>[3x]MKKILDSAKNYLNTHDKLKTACLIALELPSSSGSAATYIYLTDYFRDVTYNGILYRSGKVKSISSHKQNRQLSIGSLSFT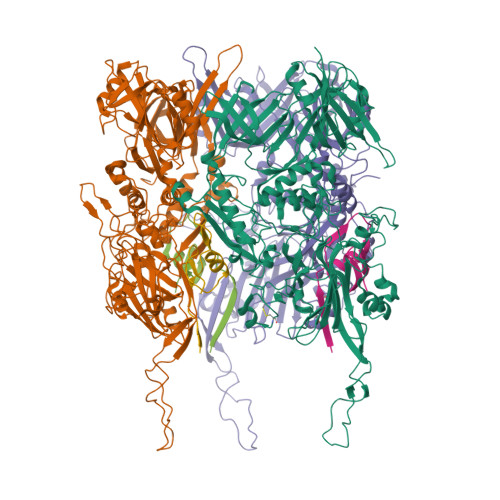ITGTAEDEVLKLVQNGVSFLDRGITIHQAIINEEGNILPVDPDTDGPLLFFRGRITGGGIKDNVNTSGIGTSVITWNCSNQFYDFDRVNGRYTDDASHRGLEVVNGTLQPSNGAKRPEYQEDYGFFHSNKSTTILAKYQVKEERYKLQSKKKLFGLSRSYSLKKYYETVTKEVDLDFNLAAKFIPVVYGVQKIPGIPIFADTELNNPNIVYVVYAFAEGEIDGFLDFYIGDSPMICFDETDSDTRTCFGRKKIVGDTMHRLAAGTSTSQPSVHGQEYKYNDGNGDIRIWTFHGKPDQTAAQVLVDIAKKKGFYLQNQNGNGPEYWDSRYKLLDTAYAIVRFTINENRTEIPEISAEVQGKKVKVYNSDGTIKADKTSLNGIWQLMDYLTSDRYGADITLDQFPLQKVISEAKILDIIDESYQTSWQPYWRYVGWNDPLSENRQIVQLNTILDTSESVFKNVQGILESFGGAINNLSGEYRITVEKYSTNPLRINFLDTYGDLDLSDTTGRNKFNSVQASLVDPALSWKTNSITFYNSKFKEQDKGLDKKLQLSFANITNYYTARSYADRELKKSRYSRTLSFSVPYKFIGIEPNDPIAFTYERYGWKDKFFLVDEVENTRDGKINLVLQEYGEDVFINSEQVDNSGNDIPDISNNVLPPRDFKYTPTPGGVVGAIGKNGELSWLPSLTNNVVYYSIAHSGHVNPYIVQQLENNPNERMIQEIIGEPAGLAIFELRAVDINGRRSSPVTLSVDLNSAKNLSVVSNFRVVNTASGDVTEFVGPDVKLAWDKIPEEEIIPEIYYTLEIYDSQDRMLRSVRIEDVYTYDYLLTYNKADFALLNSGALGINRKLRFRIRAEGENGEQSVGWATI;>MTDKLIRELLIDVKQKGATRTAKSIENVSDALENAAAASELTNEQLGKMPRTLYSIERAADRAAKSLTKMQASRGMAGITKSIDGIGDKLDYLAIQLIEVTDKLEIGFDGVSRSVKAMGNDVAAATEKVQDRLYDTNRALGGTSKGFNDTAGAAGRASRALGNTSGSARGATRDFAAMAKIGGRLPIMYAALASNVFVLQTAFESLKVGDQLNRLEQFGTIVGTMTGTPVQTLALSLQNATNGAISFEEAMRQASSASAYGFDSEQLEQFGLVARRAAAVLGVDMTDALNRVIKGVSKQEIELLDELGVTIRLNDAYENYVKQLNATSTGIKYTVDSLTTYQKQQAYANEVIAESTRRFGYLDDALKATSWEQFAANANSALRSLQQSAATYLNPVMDTLNTFLYQTKSSQMRVSAMARSASAKTTPAENVTALIENAVGAREDLDTYLKESEERVKKAQELKQQLDDLKAKQAATAPIANALTAGGIGGDESNKLVVQLTNELARQNKEIEERTKTEKVLRQAVQDTGEALLRNGKLAEQLGAKMKYADTAVPGDKGVFEVDPNNLKAVSEIQKNFDFLKKSSSDTANNIRMAASSITNAKKASSDLNSVVKAVEDTSKVTGQSADTLVKNLNLGFSSLDQMKAAQKGLSEYVTAMDKSEQNALEVAKRKDEVYNQTKDKAKAEAAAREVLLRQQQEQLTAAKALLAINPNDPEALKQVAKIETEILNTKAQGFENAKKTKDYTDKILGVDREIALLNDRTMTSTQYRLAQLRLELQLEQEKTELYSKQADGQAKVEQSRRAQAQISREIWEAEKQGTASHVSALMDALEVSQTQRNVTGQSQILTERLSILQQQLELSKGNTEEELKYRNEIYKTSAALEQLKKQRESQMQQQVGSSVGATYTPTTGLIGEDKDFADMQNRMASYDQAISKLSELNSEATAVAQSMGNLTNAMIQFSQGSLDTTSMIASGMQTVASMIQYSTSQQVSAIDQAIAAEQKRDGKSEASKAKLKKLEAEKLKIQQDAAKKQIIIQTAVAVMQAATAVPYPFSIPLMVAAGLAGALALAQASSASGMSSIADSGADTTQYLTLGERQKNVDVSMQASSGELSYLRGDKGIGNANSFVPRAEGGMMYPGVSYQMGEHGTEVVTPMVPMKATPNDQLSDGSKTTSGRPIILNISTMDAASFRDFASNNSTAFRDAVELALNENGTTLKSLGNS[3x]> HGTVASRPPVQIEELIEKPGGIIVRWCKVDDDFTAQDYRLQFRKCTANHFEDVYVGSETEFIVLHIDPNVDYQFRVCARGDGRQEWSPWSVPQTGHSTLVPHEWTTGFEGYSLSSRRNIALRNDAESSGVLYSSAPTYFCGQTLTFRVETVGQPDRRDSIGVCAERQNGYES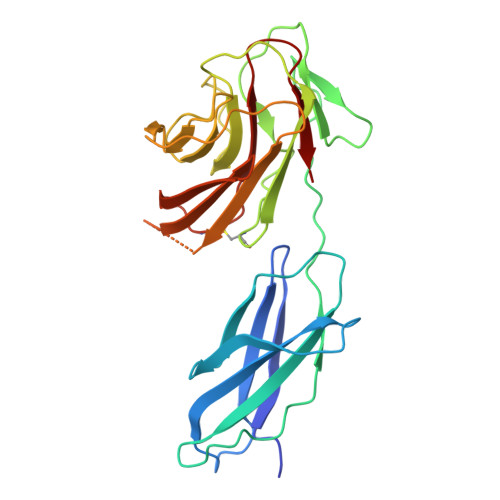LQRDQAVCISTNGAVFVNGKEMTNQLPAVTSGSTVTFDIEAVTLGTSNSHEGGNAKLRVTISSNNREVVFDWLLEQACGPLYFGCSFFYPGWKVLVF>WQENKSWNAHFTEHKSQGVVVLWNENKQQGFTNNLKRANQAFLPAGTFKIPNSLIALDLGVVKDEHQVFKWDGQTRDIATWNRDHNLITAMKYSVVPVYQEFARQIGEARMSKMLHAFDYGNEDISGNVDSFWLDGGIRISATEQISFLRKLYHNKLHVSERSQRIVKQAMLTEANGDYIIRAKTGYSTRIEPKIGWWVGWV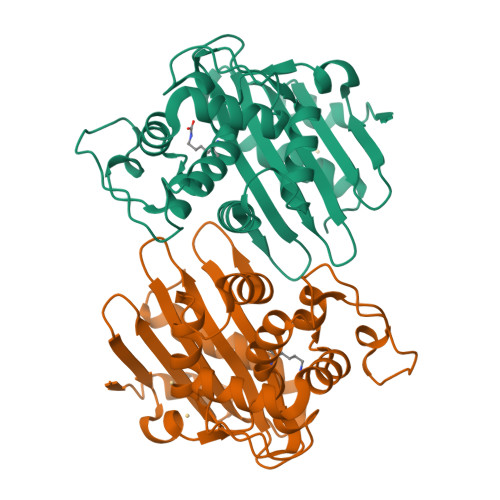ELDDNVWFFAMNMDMPTSDGLGLRQAITKEVLKQEKIIP[2x]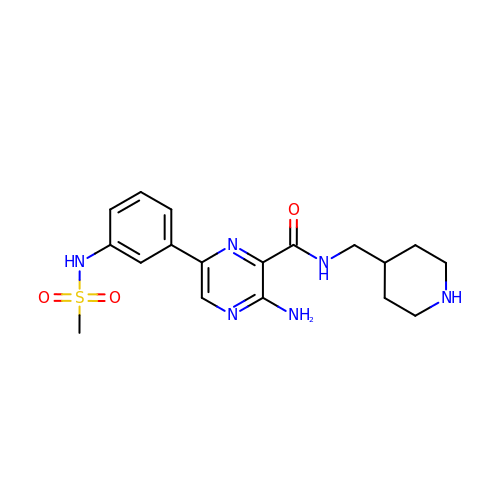3-amino-6-{3-[(methylsulfonyl)amino]phenyl}-N-(piperidin-4-ylmethyl)pyrazine-2-carboxamide | C18 H24 N6 O3 S | UCJDFWBCXROCMH-UHFFFAOYSA-N>[5x]APAAVDWRARGAVTAVKDQGQCGSCWAFSAIGNVECQWFLAGHPLTNLSEQMLVSCDKTDSGCSGGLMNNAFEWIVQENNGAVYTEDSYPYASGEGIS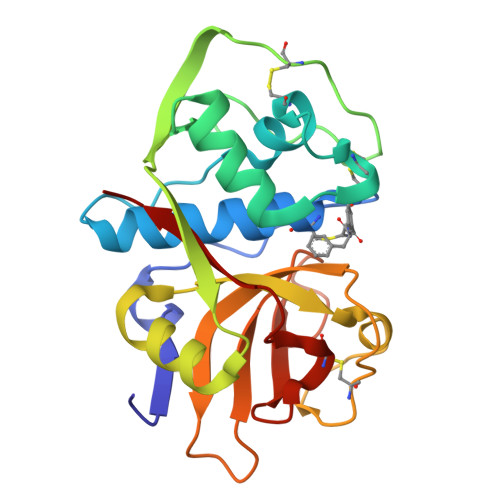PPCTTSGHTVGATITGHVELPQDEAQIAAWLAVNGPVAVAVDASSWMTYTGGVMTSCVSEQLDHGVLLVGYNDSAAVPYWIIKNSWTTQWGEEGYIRIAKGSNQCLVKEEASSAVVG> GSSVVVDTNGQPVSNGADAYYLVPVSHGHAGLALAKIGNEAEPRAVVLDPHHRPGLPVRFESPLMINIIKESYFLNIKFGPSSSDSGVWDVIQQDPIGLAVKVTDTKSLLGPF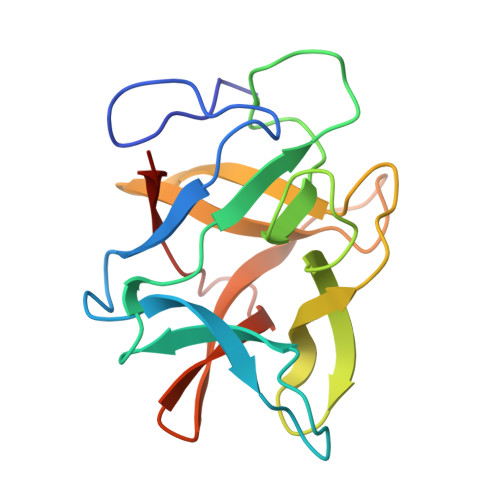KVEKEGEGYKIVYYPERGQTGLDIGLVHRNDKYYLAVKDGEPCVFKIRKAT> MKEIKLMADYHCYPLWGTTPDDFGDISPDELPISLGLKNSLEAWAKRYDAILNTDDPALSGFKSVEEEKLFIDDGYKLAELLQEELGSAYKVIYHADY;> MHHHHHHENLYFQSNAAKNSLTTKSLFKEMTIQGIKFTPENV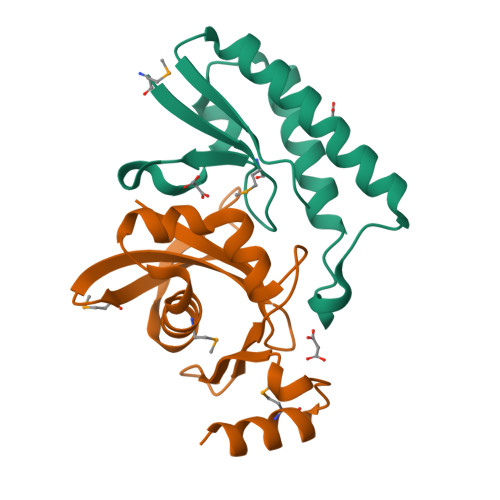VGAAKDNSGKIIFLEKGNSKSGLQHIVEEHGDQFAQIGVSEARIPDVVMKAVTDGKIVGYQGAGAGRPIYETMIDGKKYNIAVTVGSNGYVVGANLRGSVK> MSSAGSAAPPPPHTSSFGADVELPMSDWALRLQRELMSPVDPLGGLAHKDYYRDPATGYAPQYAPRDFVHGGSIAYPHMQGSGSAHDSYAAAAARRNWLEHDVESMAFMSQDARATARQLSSDAEREAFTQRHVPADRHRSAFPGNASLAAMDQLRTSGPQSDEKVYQQAILDRYRAAATSSSSSTAPGVSYTAATGLSGGELVDALAEDYAAAVDDGMDEELRIAHGLRAKERFDFKVMQRTSRVPFQGYDMDRFAAQREGRPHGAQQLPPVIPPSSME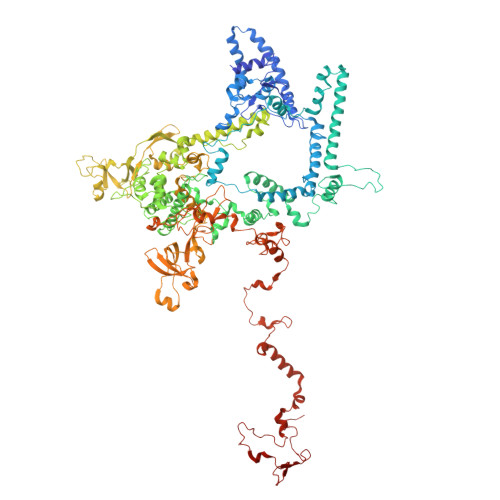EAMKNMRGGAAALLDTEAQAWQTYAQNTTSEEPKLGEALTGDVINSLHARRWSAQHAKEQARKQRFGLGRQGALVQDGGPDRRTLKKHTNDERLLDAVNFASDAYRRTITDEHVDPYVRRSTERGVGHLLTNSFDMARREDRVAHGQQDLTERNTVHYGVPIQQSIDEFVLSHRNARGERPLDYFKPFPDFRAQRLIRMYRDIEGFSLLKQRPEAFEWELFTRYRAHHQQRRELALLHGLEPVANETAAERTARRLALDELCEKTPFDPSKLHLNDDEVEIDAETLRNWFGVYVLPSPTIVESVVRAEGGALNLHLQHAADEMNTADTREHILSSRYMNRLLLFEGFQHRWNRGFTKEVAGKAPEPVIKYAQPQEVLKYFDSDERAMYQQYVQQESDAQLSEWAKVTRGRRYIAEKEQYGEVAGQGYKVPVVDVQHQETGAVLTVSSKLVEKSAAAALADKKLAGGSSSSTTSSSSMVHFDGQAYFVLPGSKRTVTPLSIRLESGESMEMTDEVFSAYPLEVSASAKYNHALNYGIGEYDYNRGNYIETQDAIWEKATADQEEGWSPATHADGLCPGLPVRARRRLAAAGEDKTGAAITGDFQRGRIVQYYRQPFFNPDPRLVTVAFYADGVVQEVPLANVMIWQRRYHGPERTVGDESRRYNPAGLRRYIDVADPNNKKLSPSSSAGAGANGAGDHFLEKYEGRLTNSVAASRYRTTKQITEIDQWNRFDTSRADNHRPLSISHRRDYVRQGYLPRYTPWEWIAIQEADQPIIHETMRTDNIGASYFFSLNRSWRYKARPHGYLRNYENEVRDMLQFVDGVTPWKQAQKIRTYWEVRQHHPMPQFNRPEVAMHRNSAGLLPSHMWEMDKKTGKVRAVKDSVRDYQTKIPVPKWVQL> MSFSSLYKTFFKRNAVFVGTIFAGAFVFQT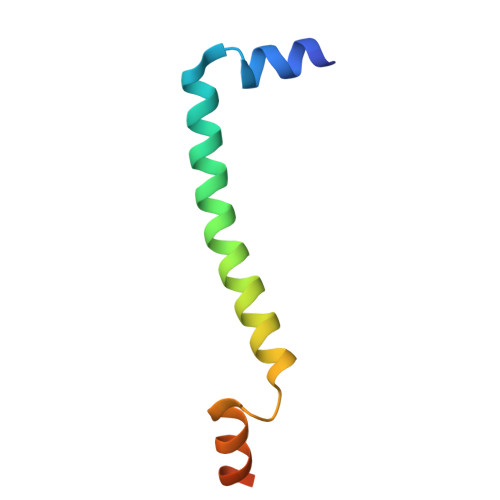VFDTAITSWYENHNKGKLWKDVKARIAAGDGDDDDE>[3x]MEKQCSKFIVSGHVQGVGFRYHTSHQGLK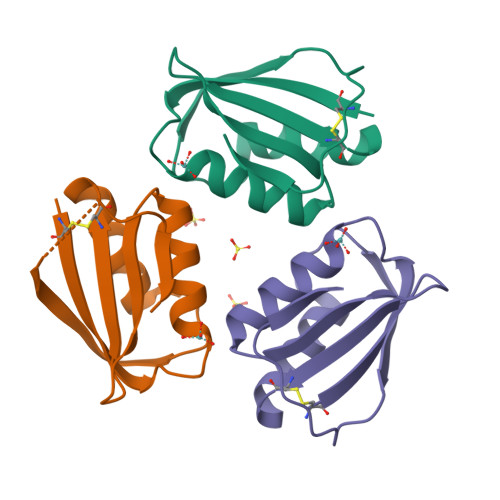LGLTGYAKNLNNGDVEVVACGTPERLEELYLWLQEGPKTASVRQVRRLSSELEHDYQGFEIL beta-D-galactopyranuronic acid | 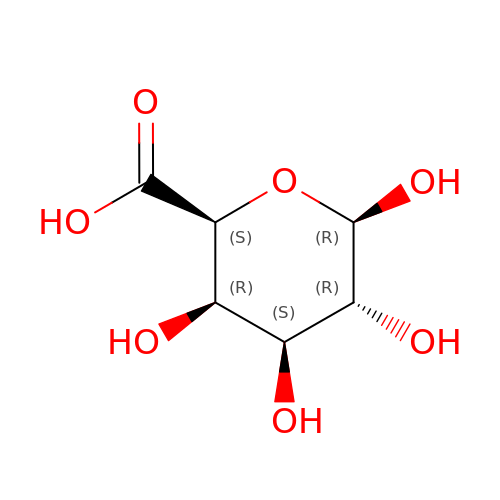C6 H10 O7 | AEMOLEFTQBMNLQ-DTEWXJGMSA-N> MMHHHHHHHHSHSGPEISRIIVDPTTGKRYSRGKTLGKGGFAKCYEMTDLTNNKVYAAKIIPHSR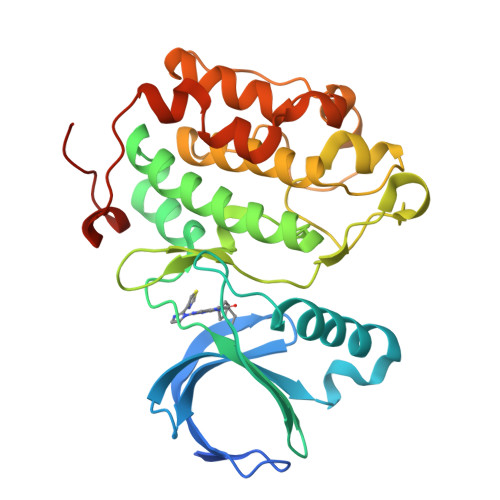VSKPHQREKIDKEIELHRILHHKHVVQFYHYFEDKENIYILLEYCSRRSMAHILKARKVLTEPEVRYYLRQIVSGLKYLHEQEILHRDLKLGNFFINESMELKVGDFGLAARLEPLEHRRRTICGTPNYLSPEVLNKQGHGAESDIWALGCVMYTMLLGRPPFETTNLKETYRSIREARYTMPSSLLAPAKHLIASMLSKNPEDRPSLDDIIRHDFFTQGFTPDRLSSSCCHTVPDFHLSSPA> MELLCCEGTRHAPRAGPDPRLLGDQRVLQSLLRLEERYVPRASYFQCVQREIKPHMRKMLAYWMLE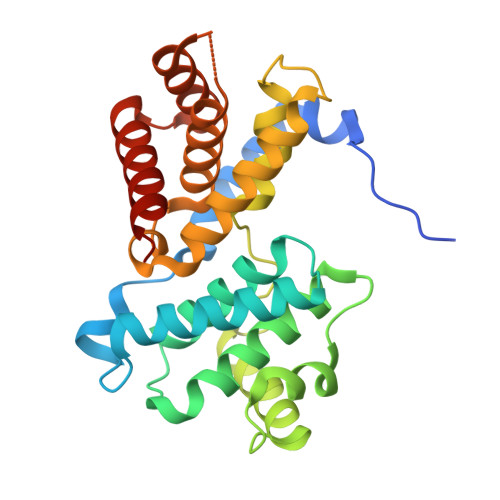VCEEQRCEEEVFPLAMNYLDRYLSCVPTRKAQLQLLGAVCMLLASKLRETTPLTIEKLCIYTDHAVSPRQLRDWEVLVLGKLKWDLAAVIAHDFLAFILHRLSLPRDRQALVKKHAQTFLALCATDYTFAMYPPSMIATGSIGAAVQGLGACSMSGDELTELLAGITGTEVDCLRACQEQIEAALRESLREAS>[2x]GSEPEPEQVIKNYTEELKVPP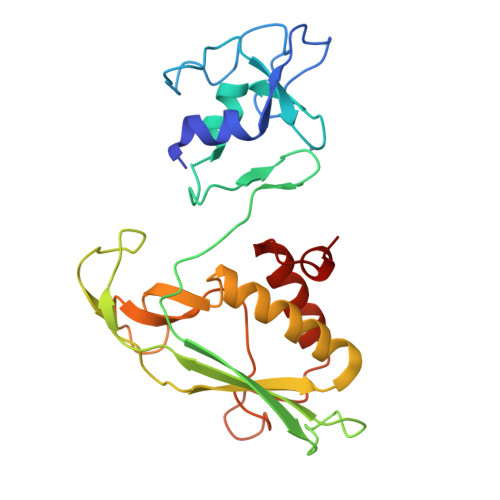DEDCIICMEKLSTASGYSDVTDSKAIGSLAVGHLTKCSHAFHLLCLLAMYCNGNKDGSLQCPSCKTIYGEKTGTQPQGKMEVLRFQMSLPGHEDCGTILIVYSIPHGIQGPEHPNPGKPFTARGFPRQCYLPDNAQGRKVLELLKVAWKRRLIFTVGTSSTTGETDTVVWNEIHHKTEMDRNITGHGYPDPNYLQNVLAELAAQGVTEDCLEQQ> MAVPFVEDWDLVQTLGEGAYGEVQLAVNRVTEEAVAVKIVDMKRAVDCPENIKKEICINAMLNHENVVKFYGHRREGNIQYLFLEYCSGGELFDRIEPDIGMPEPDAQRFFHQLMAGVVYLHGIGITHRDIKPENLLLDERDNLKISDFGLATVFRYNNRERLLNKMCGTLPYVAPELLKRREFHAEPVDVWSCGIVLTAMLAGELPWDQPSDSCQEYSDWKEKKTYLNPWKKIDSAPLALLHKILVENPSARIT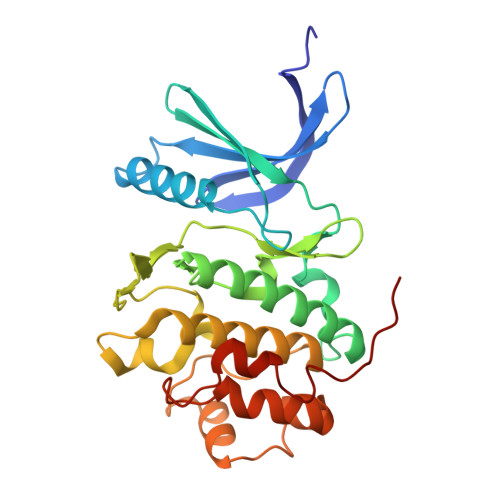IPDIKKDRWYNKPLKKGA>MAHHHHHHSSGLEVLFQGPNEQVSRSQQRGLRRVRDLCRVLQLPPTFEDTAVAYYQQAYRHSGIRAARLQKKEVLVGCCVLITCRQHNWPLTMGAICTLLYADLDVFSSTYMQIVKLLGLDVPSLCLAELVKTYCSSFKLFQASPSVPAKYVEDKEKMLSRTMQLVELANETWLVTGRHPLPVITAATFLAWQSLQPADRLSCSLARFCKLANVDLPYPASSRLQELLAVLLRMAEQLAWLRVLRLDKRSVVKHIGDLLQHRQSLVRSAFRDGTAEVETREKEPPGWGQGQGEGEVGNNSLGLPQGKRPASPALLLPPCMLKSPKRICPVPPVSTVTGDENISDSEIEQYLRTPQEVRDFQRAQAARQAATSVPNPP[2x];>[2x]MAHHHHHHSSGLEVLFQGPSGIVPQLQNIVSTVNLGCKLDLKTIALRARNAEYNPKRFAAVIMRIREPRTTALIFSSGKMVCTGAKSEEQSRLAARKYARVVQKLGFPAKFLDFKIQNMVGSCDVKFPIRLEGLVLTHQQFSSYEPELFPGLIYRMIKPRIVLLIFVSGKVVLTGAKVRAEIYEAFENIYPILKGFRKTT;>[2x]MAHHHHHHSSGLEVLFQGPGPLLVPRVKVAEDGSIILDEESLTVEVLRTKGPCVVEENDPIFERGSTTTYSSFRKNYYSKPWSNKETDMFFLAISMVGTDFSMIGQLFPHRARIEIKNKFKREEKTNGWRIDKAFQEKRPFDFDFFAHLLQKVLAEEEKRKQKSVKNHSLKEKKS

RNA polymerase III (Pol III) is the eukaryotic multisubunit DNA-dependent enzyme dedicated to the transcription of short untranslated RNAs involved in essential cellular processes, such as the entire pool of transfer RNAs, the 5S ribosomal RNA, and the spliceosomal U6 small nuclear RNA (snRNA). Transcription initiation requires the action of the TFIIIB complex, which is both required and sufficient to recruit Pol III to the promoter and to faithfully initiate transcription in yeast. In the context of such TFIIIB complexes, TBP recognizes specifically the TATA box inducing a sharp bend of the DNA, whereas the TFIIB-related factors Brf1 and Brf2, similarly to their Pol II paralog TFIIB, recognize TATA-flanking regions and interact directly with Pol III, thus effectively bridging the polymerase to its target promoters. Bdp1 contains a highly conserved SANT domain, which constitutes the major module interacting with Brf1–TBP and Brf2–TBP complexes.

Bdp1SANT could be crystallized by vapor diffusion in complex with Brf2, TBP, and a DNA fragment of 25 base pairs (bp) of the human U6 promoter (referred to as TFIIIB–DNA complex hereafter), and the X-ray structure was solved at 2.7 Å by molecular replacement. In the TFIIIB–DNA complex, Bdp1 can be schematically divided into a compact domain constituted by the Bdp1 SANT domain (helix 1–3, residues 303–348) as well as two additional C-terminal α-helices (helix 4 and 5, residues 348–382), and an N-terminal extension that forms an ordered linker (residues 286–302). Bdp1 residues 241–285, which are predicted to form a β-strand region and are essential for promoter opening in yeast, and 383–396 are not visible in the electron-density map, suggesting that in the absence of Pol III these regions are disordered. The SANT domain of Bdp1 interacts with both TBP and DNA, while a structured linker emerging at the N terminus of the SANT domain interacts with the minor groove of the DNA. The N-terminal region flanking the Bdp1 SANT domain, which we named the “Bdp1 linker” (residues 286–302), adopts an extended conformation, spanning the entire length of the minor groove of the DNA and inserting in between the two Brf2 cyclin repeats. Bdp1 residues Y299 and F294 anchor the Bdp1 linker to the major groove of the DNA through aromatic-sugar interactions with the DNA backbone. Bdp1 F294 buries into a hydrophobic cavity formed by the sugar moiety of the DNA, TBP L187, and Brf2 L146. The recognition helix (α3, residues 334–347) of Bdp1SANT contacts both sides of the major groove of the DNA, using conserved polar residues to interact with the phosphate backbone of the template and non-template DNA strands. In particular, the invariably conserved Bdp1 residue R334 forms a salt bridge with TBP residue E191, and contacts the DNA phosphate backbone of the template strand.> GGGRMKNQWQHQYFLSYSELVANFPSPEKVVSDYIKHKFSTTLPWFGWADPDNLYFIRFTQSRSNNKSYTGWDHLGKYAIETLTLTQAAIVNIGSRFDIFDEANSTAGIYKTNNADSFDETNEAKMLPSEYLYFLRDCDFSNLYNKALSDYWAENYEKFSTLLQNYYISSAYYLYKDSAISKDEYEFSIDAIFNKKNKILRYYFDVYGYYSSDMFVAMNDNKTMLFIPGATNPFIFADNITDLRDKIKALISDKNTRELFSKHFSLYDRQDGNTYLGVNSMLEQIVSGVVDTNYIMYSNKNIRERNVFESMAFSTRERSFNDGDVIIKSNAEVQRDYALNVLQTILSLSPIFDIVLPEVSIPISLGITASSVGISFDELINGDTYEERRSAIPGLATNAVLLGISFAIPFLISKAEENKLIINNLVGSDENILNKNNLGDFLEKYNISESDIPENGSLVINLKNTNVPVRLVKLNDEEGEIVAIKGSTLSGIYYEVDTETGYEILSRRVFRTEYNEKIYWTRGGGLKGGQPFNFEGLDIPVYFIDKPYSELASSVELSFVNDDSPLLFPEMDSRLPKPTPELDIKYYSSNLSSFKEDTVILMRGTTEEEAWNIANYKTAGGSNKDLEENFIEAGPQFNLSFSEYTSSINSADTASRKHFLVIIKVQVKYISNDNVLYANHWAIPDEAPVEVLAVVDRRFIFPEPPVKPKLSFIQKIANRFLTEN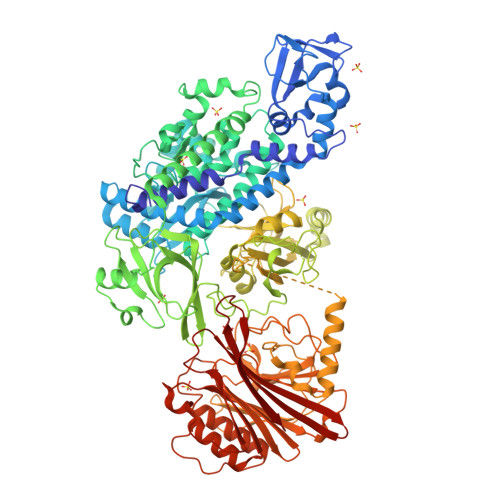VAEISSINFRRLNSGNINVLKGRGVFSSRRLREIYLRFDAANADELRPGDVYVKKTKFDSMGYDSHFYNEGIGINGAPTLNTYTGEYVADSSSQGATYWLKYNLTNETSIIKVSNSARGANGIKIALEEIEENKPVVITSGTLTGSTVVFARKGEYFYAVHTGNSESLIGFTSTSGVAKAIEVLSSLSELEVPALPDVINNNTLVEYLSDNFDSALISYSSSSLKPNSMINISRENVSTFSYYTDDIQLPSFGTSVTILVRTNDNTVVRSLSESYTMNSNSSKMVVFNVLQKDF>[2x]MRPPQFTRAQWFAIQHISLNPPRCTIAMRAINNYRWRCKNQNTFLRTTFANVV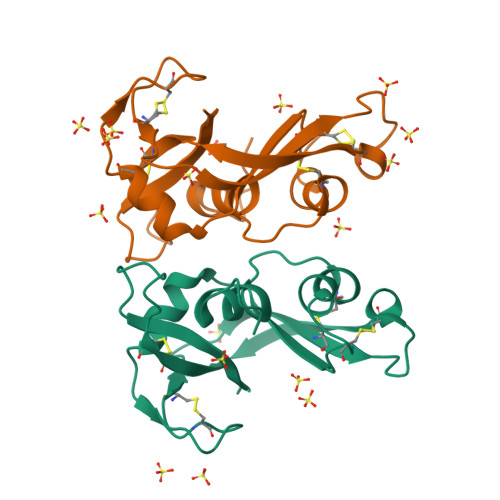NVCGNQSIRCPHNRTLNNCHRSRFRVPLLHCDLINPGAQNISNCRYADRPGRRFYVVACDNRDPRDSPRYPVVPVNLDTTI>[2x]SSVILTNYMDTQYYGEIGIGTPPQTFKVVFDTGSSNVWVPSSKCSRLYTACVYHKLFDASDSSSYKHNGTELTLRYSTGTVSGFLSQDIITVGGITVTQMFGE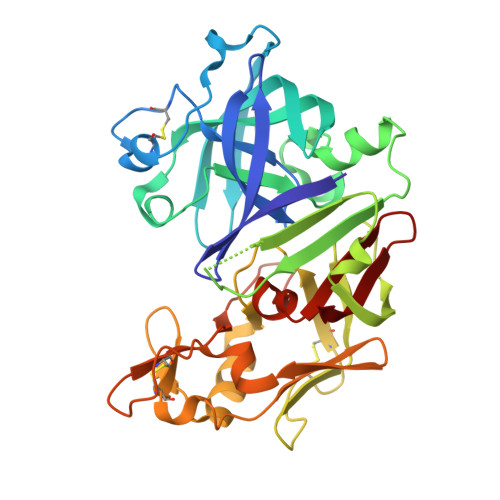VTEMPALPFMLAEFDGVVGMGFIEQAIGRVTPIFDNIISQGVLKEDVFSFYYNRDSENSQSLGGQIVLGGSDPQHYEGNFHYINLIKTGVWQIQMKGVSVGSSTLLCEDGCLALVDTGASYISGSTSSIEKLMEALGAKKRLFDYVVKCNEGPTLPDISFHLGGKEYTLTSADYVFQESYSSKKLCTLAIHAMDIPPPTGPTWALGATFIRKFYTEFDRRNNRIGFALAR2-amino-3-methyl-6-[(1S,2R)-2-(3'-methylbiphenyl-4-yl)cyclopropyl]pyrimidin-4(3H)-one | C21 H21 N3 O 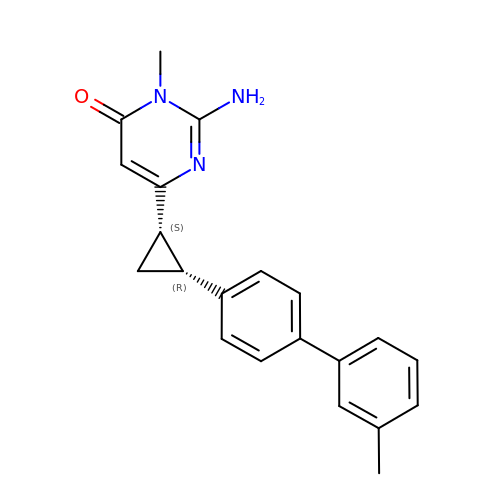| STUBOTPNCNDBOA-ROUUACIJSA-N The conserved DEAD-box RNA helicase Vasa plays diverse functions in germ cell formation and germline maintenance in animals. The core of DEAD-box RNA helicases is formed by two highly conserved RecA-like domains, often flanked by helicase-specific N-terminal and C-terminal extensions. Here, we show that LOTUS (Limkain, Oskar, and Tudor containing proteins 5 and 7) domains present in the germline proteins Oskar, TDRD5 (Tudor domain-containing 5), and TDRD7 bind and stimulate the germline-specific DEAD-box RNA helicase Vasa. Assembly of the Drosophila pole plasm is induced by the protein Oskar.

To obtain structural information regarding the LOTUS–Vasa complex and the role of LOTUS in stimulating Vasa's ATPase activity, we carried out cocrystallization experiments using the LOTUS domain of Oskar (amino acids 139–240) and the Vasa-CTD lacking the C-terminal extension (amino acids 463–623). The crystals that we obtained diffracted to 1.4 Å resolution, and the structure was solved by molecular replacement and subsequently refined against the data set to R/Rfree values of 16.9%/19.9% (see Supplemental Table S1 for data collection and model refinement statistics). The crystal structure consists of one LOTUS dimer and two molecules of Vasa-CTD, each one bound to a LOTUS monomer on the side opposite to the dimerization interface. Hence, Vasa binding does not affect dimerization of the LOTUS domain, which is consistent with the experimentally determined 1:1 stoichiometry of the LOTUS–Vasa complex. The interface area of one LOTUS monomer–Vasa-CTD subcomplex measures 1080 Å2 (PISA analysis). In the complex, the LOTUS domain is contacted mainly via the α2 helix of the Vasa-CTD. Conversely, the Vasa-CTD is contacted by two helices of the LOTUS domain: the α2 helix, which is part of the trihelical bundle of the winged HTH (wHTH) core, and the α5 helix, which is positioned at the LOTUS domain C terminus. Interestingly, although one of our previously obtained crystal structures of the LOTUS domain alone also contained the C-terminal extension (α5 helix in the cocrystal), the extension did not adopt a particular secondary structure but most likely was disordered (Jeske et al. 2015). This suggests that the LOTUS domain C-terminal extension forms an α helix upon interaction with Vasa. In Vasa, we identified two point mutations in the α2 helix of the CTD (F504E and F508E), each of which prevents the Vasa–eLOTUS interaction in GST pull-down assays. In the eLOTUS-bound CTD, the conformation of these motifs resembles that observed in DEAD-box helicases in their open state, suggesting that the conformation of the open state CTD does not change upon eLOTUS domain binding.

>GPLGSMTIIESNYISVREEYPDIDSEVRAILLSHAQNGITISSIKSEYRKLTGNPFPLHDNVTDFLLTIPNVTAECSESGKRIFNLKASLKNGHLLDMVLNQKERTS[2x];>[2x]GHSDVKQTIYEVNKYAKRSKLIEILSEQADGTIVFVETKRGADFLASFLSEKEFPTTSIHGDRLQSQREQALRDFKNGSMKVLIATSVASRGLDIKNIKHVINYDMPSKIDDYVHRIGRTGRVGNNGRATSFFDPEKDRAIAADLVKILEGSGQTVPDFLRTC>[2x]MELWLVRHGETMWNREGRLLGWTDLPLTAEGEAQARRLKGALPSLPAFSSDLLRARRTAELAGFSPRLYPELREIHFGALEGALWETLDP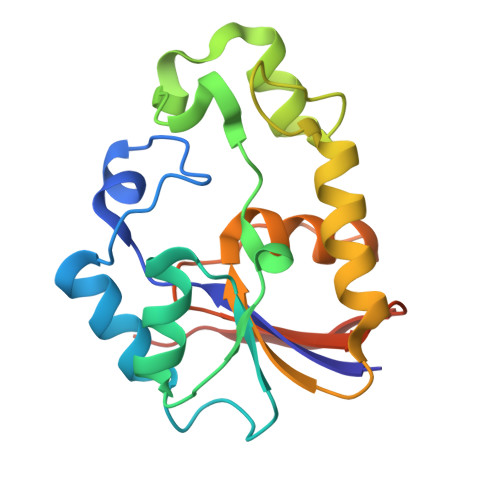RYKEALLRFQGFHPPGGESLSAFQERVFRFLEGLKAPAVLFTHGGVVRAVLRALGEDGLVPPGSAVAVDWPRRVLVRLALDGEEATG> AMNLIPEDGLPPILISTGVKGDYAVEEKPSQISVMQQLEDGGPDPLVFVLNANLLSMVKIVNYVNRKCWCFTTKGMHAVGQSEIVILLQCLPDEKCLPKDIFNHFVQLYRDALAGNVVSNLGHSFFSQSFLGSKEHGGFLYVTSTYQSLQDLVLPTPPYLFGILIQKWETPWAKVFPIRLMLRLGAEYRLYPCPLFSVRFRKPLFGETGHTIMNLLADFRNYQYTLPVVQGLVVDMEVRKTSIKIPSNRYNEMMKAMNKSNEHVLAGGACFNEKADSHLVCVQNDDGNYQTQAISIHNQPRKVTGASFFVFSGALKSSSGYLAKSSIVEDGVMVQITAENM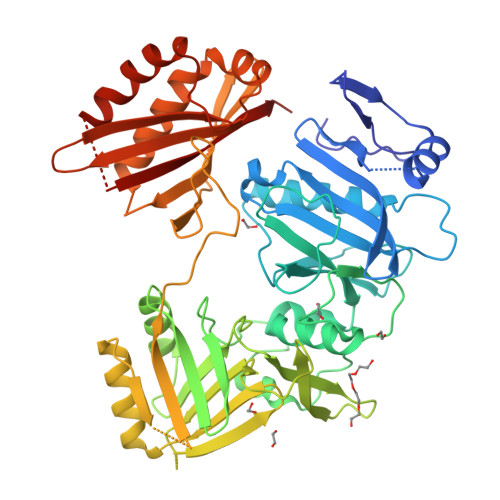DSLRQALREMKDFTITCGKADAEEPQEHIHIQWVDDDKNVSKGVVSPIDGKSMETITNVKIFHGSEYKANGKVIRWTEVFFLENDDQHNCLSDPADHSRLTEHVAKAFCLALCPHLKLLKEDGMTKLGLRVTLDSDQVGYQAGSNGQPLPSQYMNDLDSALVPVIHGGACQLSEGPVVMELIFYILENIV>[4x]GPGLKQKIVIKVAMEGNNCRSKAMALVASTGGVDSVALVGDLRDKIEVVGYGIDPIKLISALRKKVGDAELLQVEQAKED;>[2x]METGNKYIEKRAIDLSRERDPNFFDNPGIPVPECFWFMFKNNVRQDDGTCYSSWKMDMKVGPNWVHIKSDDNCNLSGDFPPGWIVLGKKRPGF

The rice NLR receptor Pik-1 binds the Magnaporthe oryzae effector AVR-Pik through an integrated heavy metal-associated (HMA) domain. The sensor NLR Pik-1 contains an integrated HMA domain between the CC and NB-ARC domains (Maqbool et al., 2015). Direct binding of AVR-Pik to the HMA domain is required to activate Pik-mediated immunity. However, the stealthy alleles AVR-PikC and AVR-PikF avoid interaction with Pik-HMA and evade host defenses.

The Asp67 and Lys78 polymorphisms that distinguish AVR-PikC and AVR-PikF from AVR-PikE and AVR-PikA, respectively, are located at interface 2. The crystal structure of the OsHIPP19-HMA/AVR-PikF complex revealed additional hydrogen bond interactions at interface 3 relative to integrated HMAs in the complex with AVR-Pik variants. The corresponding residue in all described Pik-1 HMA domains is serine, and while the hydroxyl group of the serine side chain only forms an intramolecular hydrogen bond within the HMA domain, the bulkier OsHIPP19Glu72 side chain extends across the interface and forms a direct hydrogen bond with the effector. By contrast, PikpSNK-EKE-HMA bound to both AVR-PikC and AVR-PikF with higher apparent affinity (larger %Rmax) than PikpNK-KE-HMA. By determining the crystal structures of the Pikp-HMASNK-EKE/AVR-PikC and Pikp-HMASNK-EKE/AVR-PikF complexes, we confirmed the formation of new contacts across the HMA/effector interface that likely account for the expanded recognition profile to AVR-PikC and AVR-PikF. Crystals were obtained in several conditions in the Morpheus screen (Molecular Dimensions), and X-ray diffraction data were collected at the Diamond Light Source (Oxford, UK) to a resolution of 2.15 Å (Pikp-HMANK-KE/AVR-PikC), 2.05 Å (Pikp-HMASNK-EKE/AVR-PikC), and 2.2 Å (Pikp-HMASNK-EKE/AVR-PikF). Interface analysis performed with qtPISA identified 15 hydrogen bonds and nine salt bridges between Pikp-HMASNK-EKE and AVR-PikC, and 16 hydrogen bonds and 11 salt bridges between Pikp-HMASNK-EKE and AVR-PikF, compared to the 12 hydrogen bonds and eight salt bridges mediating the interaction between Pikp-HMANK- KE and AVR-PikC. Inspection of the structures revealed that the side chain of Glu258 does indeed extend across the interface, forming direct hydrogen bonds with the backbone of the effectors. This single mutation also supports additional hydrogen bonds at the interface between AVR-PikC (or AVR-PikF) and residues comprising β4 of the HMA domain.> ITCYKTPIITSETCAPGQNLCYTKTWCDAWCGS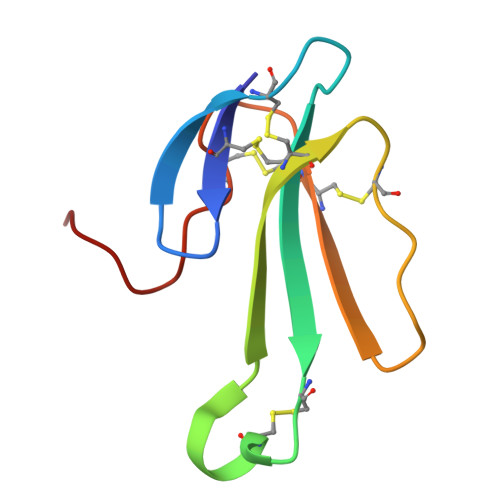RGKVIELGCAATCPTVESYQDIKCCSTDNCNPHPKQKRP>MTADELVFFVNGKKVVEKNADPETTLLVYLRRKLGLCGTKLGCGEGGCGACTVMISKYDRLQNKIVHFSVNACLAPICSLHHVAVTTVEGIGNTQKLHPVQERIARSHGSQCGFCTPGIVMSMYTLLRNQPEPTVEEIENAFQGNLCRCTGYRPILQGFRTFAKDGGCCGGSGNNPNCCMNQTKDQTVSLSPSLFNPEDFKPLDPTQEPIFPPELLRLKDTPQKKLRFEGERVTWIQASTMEELLDLKAQHPDAKLVVGNTEIGIEMKFKNMLFPLIVCPAWIPELNSVVHGPEGISFGASCPLSLVESVLAEEIAKLPEQKTEVFRGVMEQLRWFAGKQVKSVASIGGNIITASPISDLNPVFMASGAKLTLVSRGTRRTVRMDHTFFPGYRKTLLRPEEILLSIEIPYSKEGEFFSAFKQASRREDDIAKVTSGMRVLFKPGTIEVQELSLCFGGMADRTISALKTTPKQLSKSWNEELLQSVCAGLAEELQLAPDAPGGMVEFRRTLTLSFFFKFYLTVLQKLGRADLEDMCGKLDPTFASATLLFQKDPPANVQLFQEVPKDQSEEDMVGRPLPHLAANMQASGEAVYCDDIPRYENELSLRLVTSTRAHAKITSIDTSEAKKVPGFVCFLTAEDVPNSNATGLFNDETVFAKDEVTCVGHIIGAVVADTPEHAQRAARGVKITYEDLPAIITIQDAINNNSFYGSEIKIEKGDLKKGFSEADNVVSGELYIGGQEHFYLETNCTIAVPKGEAGEMELFVSTQNTMKTQSFVAKMLGVPDNRIVVRVKRMGGGFGGKETRSTVVSTALALAAHKTGRPVRCMLDRDEDMLITGGRHPFLAKYKVGFMKTGTVVALEVAHFSNGGNTEDLSRSIMERALFHMDNAYKIPNIRGTGRICKTNLPSNTAFRGFGGPQGMLIAEYWMSEVAITCGLPAEEVRRKNMYKEGDLTHFNQKLEGFTLPRCWDECIASSQYLARKREVEKFNRENCWKKRGLCIIPTKFGISFTLPFLNQGGALVHVYTDGSVLLTHGGTEMGQGLHTKMVQVASRALKIPTSKIHISETSTNTVPNTSPTAASASADLNGQGVYEACQTILKRLEPFKKKKPTGPWEAWVMDAYTSAVSLSATGFYKTPNLGYSFETNSGNPFH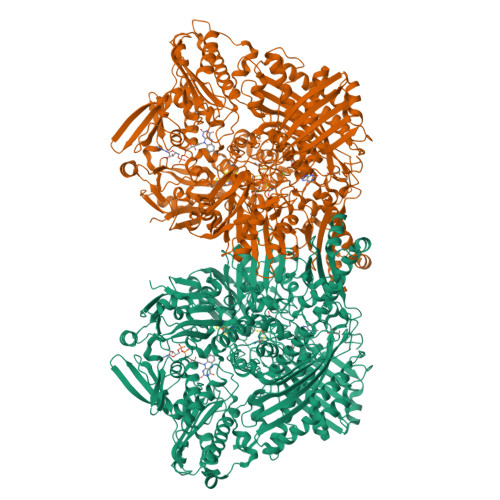YFSYGVACSEVEIDCLTGDHKNLRTDIVMDVGSSLNPAIDIGQVEGAFVQGLGLFTMEELHYSPEGSLHTRGPSTYKIPAFGSIPIEFRVSLLRDCPNKRAIYASKAVGEPPLFLASSIFFAIKDAIRAARAQHGDNAKQLFQLDSPATPEKIRNACVDQFTTL[2x]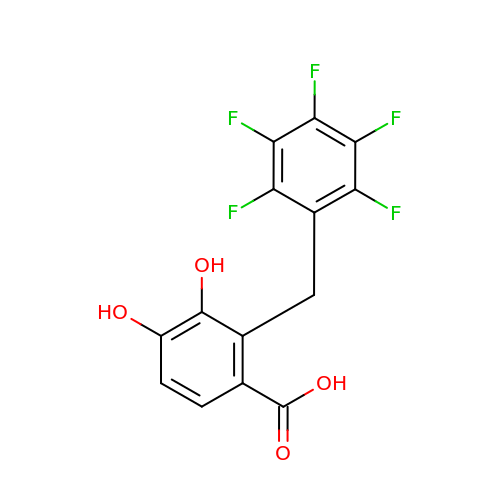3,4-DIHYDROXY-2-[(2,3,4,5,6-PENTAFLUOROPHENYL)METHYL]BENZOIC ACID | C14 H7 F5 O4 | OKFLUGFRGVSRHK-UHFFFAOYSA-N> SIWSRVVQFGTGWGFWVSGHVFITAKHVAPPKGTEIFGRKPGDFTVTSSGDFLKYYFTSAVRPDIPAMVLENGCQEGVVASVLVKRASGEMLALAVRMGSQAAIKIGSAVVHGQTGMLLTGSNAKAQDLGTIPGDAGCPYVYKKGNTWVVIGVHVAATRSGNTVIAATHGEPTLEA

Whereas ORF2, ORF3 and ORF4 each encode single proteins, ORF1 codes for a large polyprotein (∼190 kDa) that is processed by the virally-encoded protease at five specific sites to release the six ‘mature’ non-structural proteins (NS1/2–NS7)—and an array of functional precursors—that are required for virus replication. The viral NS6 protease present within the C-terminal half of the polyprotein performs all the processing, including its own autocatalytic release from the precursor (Liu, Clarke & Lambden, 1996; Belliot et al., 2003; Sosnovtsev et al., 2006; Scheffler et al., 2007). Norovirus NS6 is a cysteine protease with a chymotrypsin-like fold: two β-barrel domains separated by a cleft that contains a Cys-His-Asp/Glu catalytic triad similar in arrangement to the Ser-His-Asp triad characteristic of serine proteases. To this end we extended an inactive MNV NS6 construct (which incorporates a C139A mutation to knock out the active site nucleophile) by adding residues from NS7, which is immediately downstream in the polyprotein.

We made three constructs, NS6 1′, NS6 2′ and NS6 4′, which were extended by 1, 2 and 4 residues respectively, generating proteases that contain substrates that correspond to P4–P1′, P4-P2′ and P4-P4′ of the NS6–NS7 cleavage junction. MNV NS6 4′ crystallised in space group C2 but in a unit cell that is very different from the C2 crystals obtained with MNV NS6 1′ and that has only one molecule in the asymmetric unit. The electron density was sufficient to build a model that starts at residue 4 and ends at residue 179. Although the extended C-terminus of NS6 once again reaches between loops bII-cII and eII-fII of its near neighbour, the relation between the two molecules does not involve two-fold or quasi two-fold symmetry. However, no specific contacts are made by the C-terminal peptide with the substrate binding site.> HHHVPLTFDLPFEELLTYPGRTPRPADHDEYWDRGLADLAAVPADVVIEPAEFTTPLARCSHLWFTGTGGVRVHAKLLRPVAPVEPHPALLQFHGYTGNSGDWSSRLHYVALGYTVAALDCRGQAGLSVGEAPVENWSMASYLLRGIDDDAADNLALRHLFLDTARL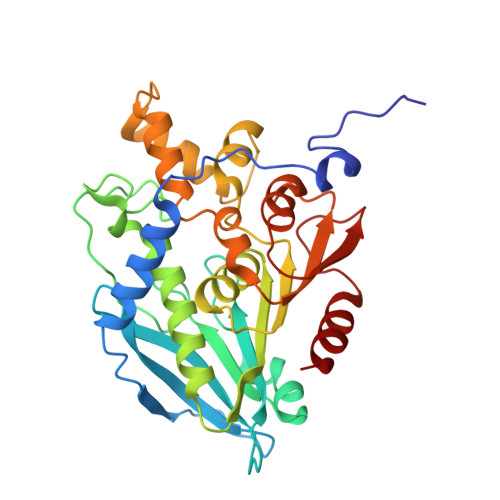AQIVLAMDDVDPDRVAATGYSQGGGLTLACAALEPRIRLAAPVYPFLCDFRRAWEMDLEKGPYNEITTYFRARDPRHLREEEIFSRLGYVDVQHLAPRVRAEVLMTVSLADKICPPSTQFAAYNKLGGPKDYRLYPDFAHETLPGTDDAIFTFLQGL>GGGAUCUGUCACCCCAUUGAUCGCCUUCGGGCUGAUCUGGCUGGCUAGGCGGGUCCC[2x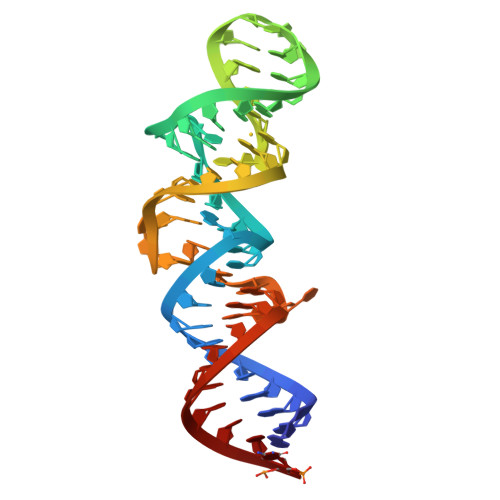]> NANDNVVIVGTGLAGVEVAFGLRASGWEGNIRLVGDATVIPHHLPPLSKAYLAGKATAESLYLRTPDAYAAQNIQLLGGTQVTAINRDRQQVILSDGRALDYDRLVLATGGRPRPLPVASGAVGKANNFRYLRTLEDAECIRRQLIADNRLVVIGGGYIGLEVAATAIKANMHVTLLDTAARVLERVTAPPVSAFYEHLHREAGVDIRTGTQVCGFEMSTDQQKVTAVLCEDGTRLPADLVIAGIGLIPNCELASAAGLQVDNGIVINEHMQTSDPLIMAVGDCARFHSQLYDRWVRIESVPNALEQARKIAAILCGKVPRDEAAPWFWSDQYEIGLKMVGLSEGYDRIIVRGSLAQPDFSVFYLQ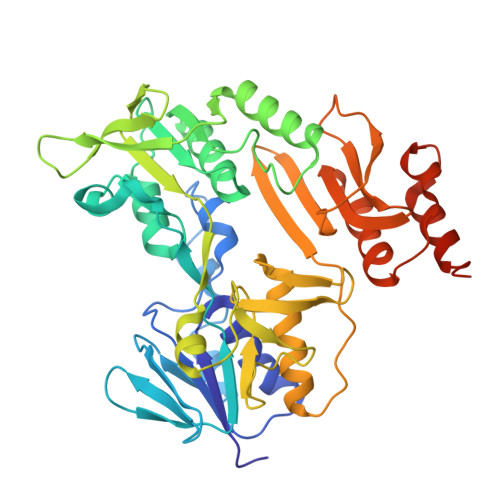GDRVLAVDTVNRPVEFNQSKQIITDRLPVEPNLLGDESVPLKEIIAAAKAELSSAKAELSSAPRHHHHHH> TIGPVTPLDASDFALDIRMPGVTPKE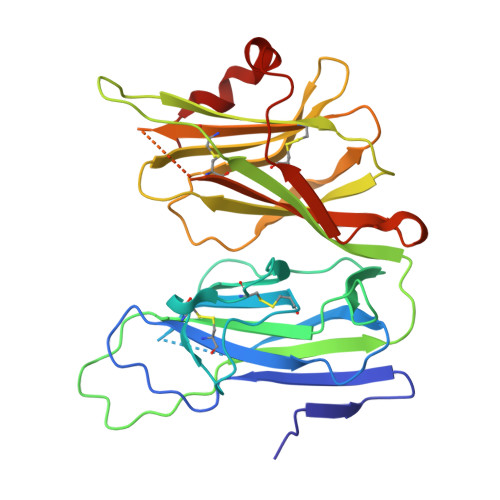SDTYFCMSMRLPVDEEAFVIDFKPRASMDTVHHMLLFGCNMPSSTGSYWFCDEGTCTDKANILYAWARNAPPTRLPKGVGFRVGGETGSKYFVLQVHYGDISAFRDNHKDCSGVSVHLTRVPQPLIAGMYLMMSVDTVIPPGEKVVNADISCQYKMYPMHVFAYRVHTHHLGKVVSGYRVRNGQWTLIGRQNPQLPQAFYPVEHPVDVTFGDILAARCVFTGEGRTEATHIGGTSSDEICNLYIMYYMEAKYALSFMTCTKNVAPDMFRTIPAEANIPIP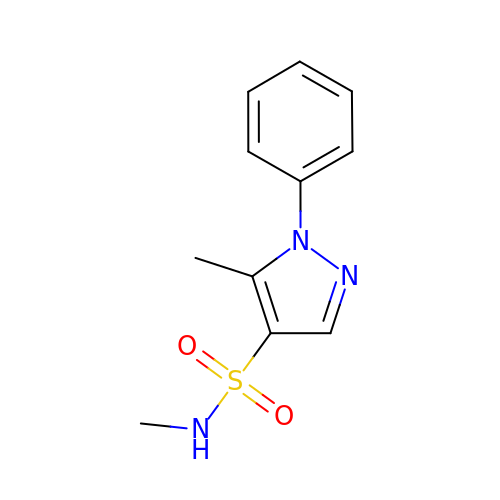~{N},5-dimethyl-1-phenyl-pyrazole-4-sulfonamide | C11 H13 N3 O2 S | GGFXNMABROEKLJ-UHFFFAOYSA-N>SSQPDPTPEQLNKSSQFTGVMGNLRCLYDNHFVEGTNVRSTGQLLQHDLIFPIKDLKLKNYDSVKTEFNSKDLATKYKNKDVDIFGSNYYYNCYYSEGNSCKNAKKTCMYGGVTEHHRNQIEGKFPNITVKVYEDNENILSFDITTNKKQVTVQELDCKTRKILVSRKNLYEFNNSPYETGYIKFIESSGDSFWYDMMPAPGAIFDQSKYLMLYNDNKTVSSSAIAIEVH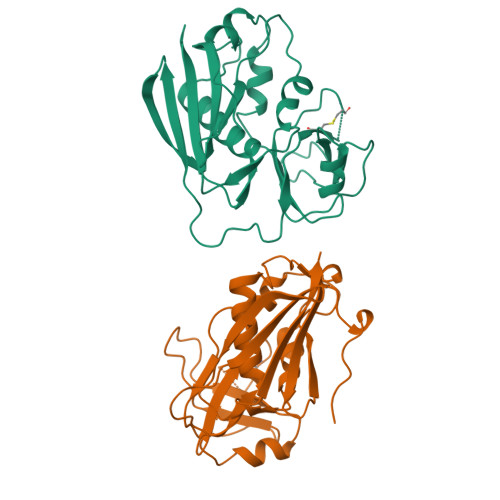LTKK[2x]>GPGSHVEEYVVEKILGKRFVNGRPQVLVKWSGFPNENNTWEPLENVGNCMKLVSDFESEVFRLHRKAAAKSVGKS[3x];>KQ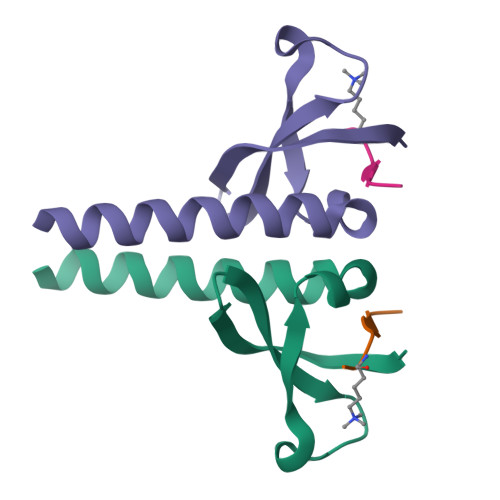TARKSTGGK[3x]>[4x]MHHHHHHHHHHLEVLFQGPSEFPMAQSNIIAGMDLNRLDRIAEHLDRAYLHPGKLAGTMTLVARRGEVVYCQAQGLRDVERQLPVERDTLFRIYSMTKPITSIALMQLYEQGRFLLDEPVHKYIPTWKNLRVYKTGSHPQMLTTAPQRPMTIRDLLTHQSGLTYGFMNRTNVDAAYRSLKLDGGPGHTLDRLIDELARLPLEFSPGTAWNY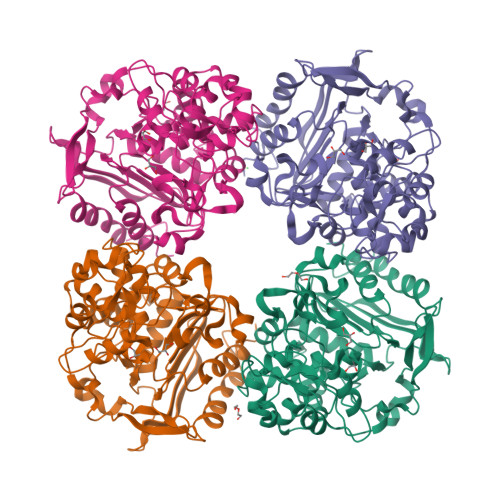SVATDVCGYLVQLLSGMSLDDYFSKHIFQPLGMPDTFFTVPAEKLSRFAACYEYQPGDSFSLQDDPQGSAFAKAHGYLSGGGGLVSCVDDYYRFAQALANGGELDGARIIGRKTLEFMRMNHLPDNKGLPDVAIGSFSETPYDGTGFGLGFSVKLDVAKSQTVGSVGEYGWGGMASTNFFIDPEEDLLMVFMTQLIPSSTYAVRQELRAIINGALVDA> MGHHHH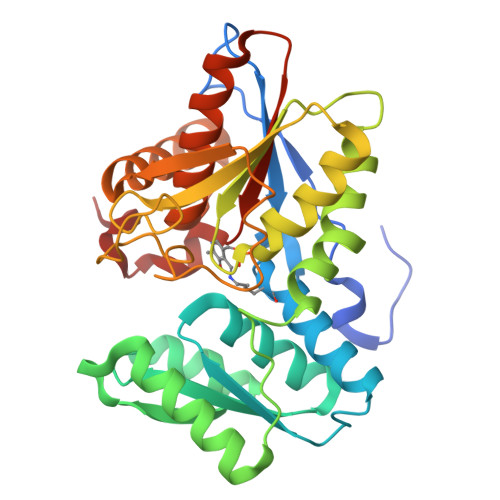HHMAQKPVDNITQIIGGTPVVKLRNVVDDNAADVYVKLEYQNPGGSVKDRIALAMIEKAEREGKIKPGDTIVEPTSGNTGIGLAFVCAAKGYKAVFTMPETMSQERRNLLKAYGAELVLTPGSEAMKGAIKKAKELKEEHGYFEPQQFENPANPEVHELTTGPELLQQFEGKTIDAFLAGVGTGGTLSGVGKVLKKEYPNIEIVAIEPEASPVLSGGEPGPHKLQGLGAGFIPGTLNTEIYDSIIKVGNDTAMEMSRRVAKEEGILAGISSGAAIYAAIQKAKELGKGKTVVTVLPSNGERYLSTPLYSFDD> MGHHHHHHHHHHSSGHIEGRHMDINGVLLLDKPQGMSSNDALQKVKRIYNANRAGHTGALNPLATGMLPICLGEATKFSQYLLDSDKRYRVIARLGQRTDTSDADGQIVEERPVTFSAEQLAAALDTFRGDIEQIPSMYSALKYQGKKLYEYARQGIEVPREARPITVYELLFIRHEGNELELEIHCSKGTYIRTIIDDLGEKLGCGAHVIYLRRLAVSKYPVERMVTLEHLRELVEQAEQQDIPAAELLDPLLMPMDSPASDYPVVNLPLTSSV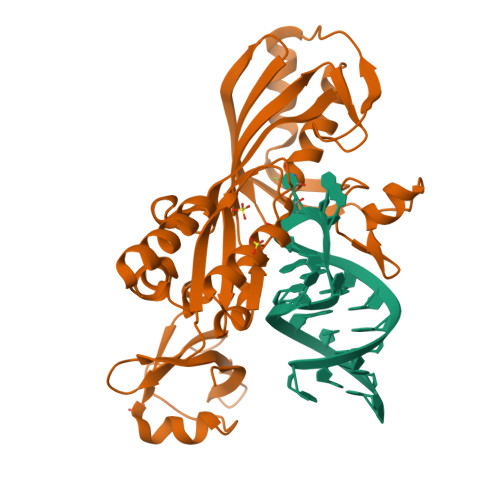YFKNGNPVRTSGAPLEGLVRVTEGENGKFIGMGEIDDEGRVAPRRLVVEYPA> MASMEEPPLLPGENIKDMAKDVTYICPFTGAVRGTLTVTNYRLYFKSMERDPPFVLDASLGVINRVEKIGGASSRGENSYGLETVCKDIRNLRFAHKPEGRTRRSIFENLMKYAFPVSNNLPLFAFEYKEVFPENGWKLYDPLLEYRRQGIPNESWRITKINERYELCDTYPALLVVPANIPDEELKRVASFRSRGRIPVLSWIHPESQATITRCSQPMVGVSGKRSKEDEKYLQAIMDSNAQSHKIFIFDARPSVNAVANKAKGGGYESEDAYQNAELVFLDIHNIHVMRESLRKLKEIVYPNIEETHWLSNLESTHWLEHIKLILAGALRIADKVESGKTSVVVHSSDGWDRTAQLTSLAML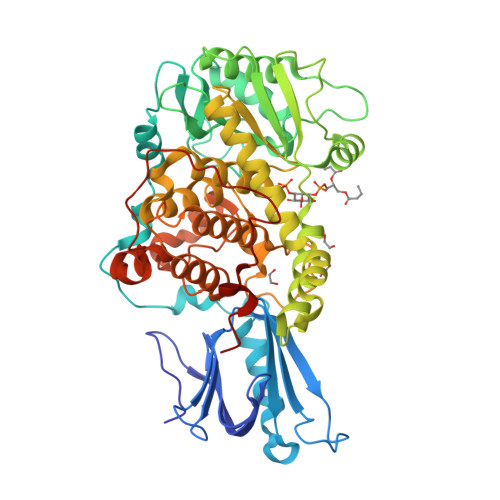MLDGYYRTIRGFEVLVEKEWLSFGHRFQLRVGHGDKNHADADRSPVFLQFIDCVWQMTRQFPTAFEFNEYFLITILDHLYSCLFGTFLCNSEQQRGKENLPKRTVSLWSYINSQLEDFTNPLYGSYSNHVLYPVASMRHLELWVGYYIRWNPRAAALEHHHHHH>STSRGMITDRSGRPLAVSVPVGGGESRRYYPSGEVTAHLIGFTNVDSQGIEGVEKSFDKWLTGQGGGAAHNLALSIDERLQALVYRELNNAVAFNKAESGSAVLVDV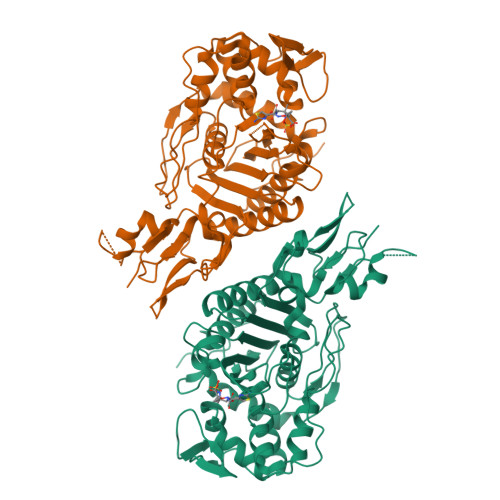NTGEVLAMANSPSYNPNNFAGTAKDTMRNRAITDVFEPGSTVKPMVVMTALQRGIVNENTVLNTVPYRINGHEIKDVARYSELTLTGVLQKSSNVGVSKLALAMPSSALVDTYSRFGLGKATNLGLVGERSGLYPQKQRWSDIERATFSFGYGLMVTPLQLARVYATIGSYGIYRPLSITKVDPPVPGERVFPESLVRTVVHMMESVALPGGGGVKAAIKGYRIAIKTGTAKKVGPDGRYINKYIAYTAGVAPASHPRFALVVVINDPQAGKYYGGAVSAPVFGAIMGGVLRTMNIEPDALAT[2x]> GCGCGCG;> TC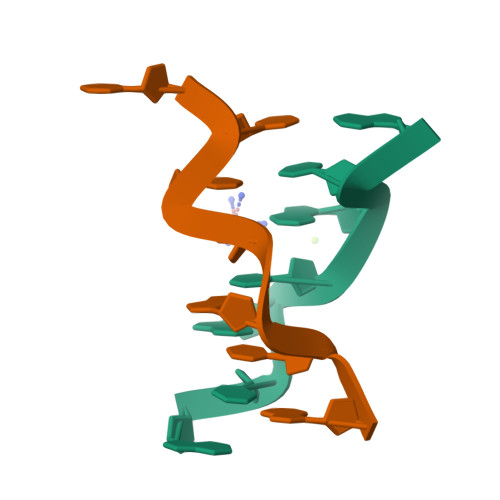GCGCG>MDEFELIKRNTSEIISEEELREVLKKDEKSASIGFEPSGKIHLGHYLQIKKMIDLQNAGFDIIIALADLMAYLNQKGELDEIRKIGDYNKKVFEAMGLKAKYVYGSEFQLDKDYTLNVYRLALKTTLKRARRSMELIAREDENPKVAEVIYPIMQVNSIHYEGVDVAVGGMEQRKIHMLARELLPKKVVCIHNPV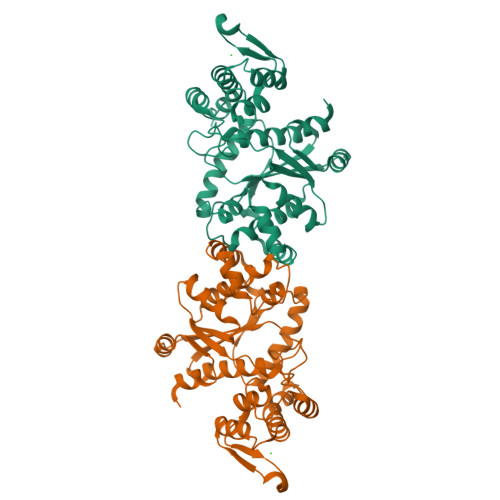LTGLDGEGKMSSSKGNFIAVDDSPEEIRAKIKKAYCPAGVVEGNPIMEIAKYFLEYPLTIKRPEKFGGDLTVNSYEELESLFKNKELHPMRLKNAVAEELIKILEPIRKRLSAHHHHHH[8x]> PNSMKNIESLFDYSAGQFEFIDHLLTMGVGVHFAALIFFLVVSQFVAPKYRIATALSCIVMVSAGLILNSQAVMWTDAYAYVDGSYQLQDLTFSNGYRYVNWMADIPCLLLQLLIVLNLKGKELFSTATWLILAAWGMIITGYVGQLYEVDDIAQLMIWGAVSTAFFVVMNWIVGTKIFKNRATMLGGTDSTITKVFWLMMFAWTLYPIAYLVPAFMNNADGVVLRQLLFTIADISSKVIYGLMITYIAIQQSAAAGYVPAQQALGRIGMDSKAA

In contrast, the NTQ rhodopsin functions as a light-driven inward chloride pump (called ClR). Here we report the atomic crystal structure of ClR from the flavobacterium Nonlabens marinus S1-08T. The structure reveals two chloride ion-binding sites, one at the active centre of the pump and the other on a loop in the cytoplasmic side, suggesting the pathway of chloride ion movement in ClR. The ClR structure comprises a short N-terminal helix, seven transmembrane helices (TM A–TM G), a C-terminal helix and three loops connecting the transmembrane helices on both extracellular and cytosolic sides.

Because Asn98 and Thr102 are the only residues of ClR directly interacting with Cl−-I, we investigated whether the interaction between Asn98 or Thr102 and Cl−-I is essential for the chloride-pumping activity of ClR. We expressed several ClR mutants (N98A, N98D and N98L for Asn98; and T102D, T102N and T102V for Thr102) in Escherichia coli cells. Of the mutants, T102N retained ∼70% of its pumping activity compared with the wild-type protein, whereas T102D completely lost its pumping activity. T102N's absorption spectra showed a blue shift in 1.5 M NaCl (λmax from 562 to 529 nm) suggesting that a chloride ion can bind at PSB but T102D's absorption spectra did not change in 1.5 M NaCl. We crystallized T102N and T102D proteins and collected diffraction data. In the T102D crystal structure, on the contrary, the side chain of the introduced Asp interacts with both PSB and Asn98, preventing the binding of a chloride at the Cl−-I site. Taken together, these results show that the direct hydrogen bond between Asn98/Thr102 (Asn98 and Thr102) and Cl−-I is crucial for the binding of Cl−-I, as well as for the chloride-pumping activity of ClR. We thus speculate that the decreased ion translocation might have arisen from the weakened binding affinity between the mutant ClRs and chloride.PTEROIC ACID | C14 H12 N6 O3 | 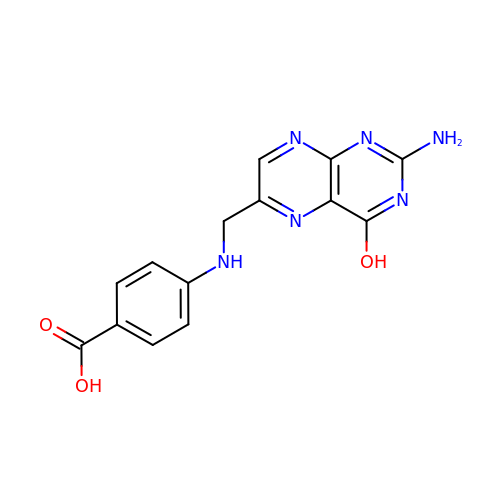JOAQINSXLLMRCV-UHFFFAOYSA-N>SNAMDAEQRLAKIIASGDECDRATVEELYDRLAPVPVDFMLGTWRGGIFDRGDALAGMLLGMNWYGKRFIDRDHVEPLLCRSPD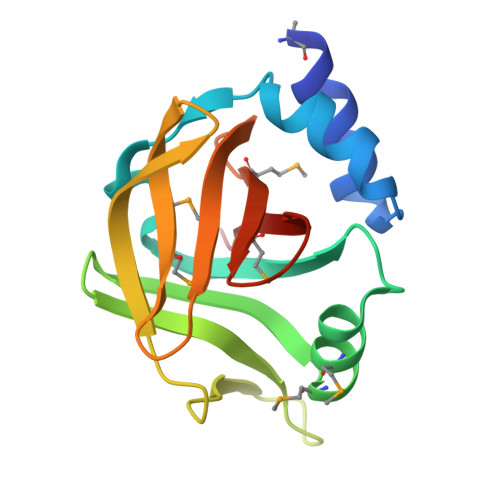GSIYSYEKLGLARLREVALRGTVSAAMIYDKQPIIDHFRRVNDDMVVGAMDAKGQPDILYFHLTRER[2x]> AHVVTDNCIKCKYTDCVEVCPVDCFYEGPNFLVIHPDECIDCALCEPECPAQAIFSED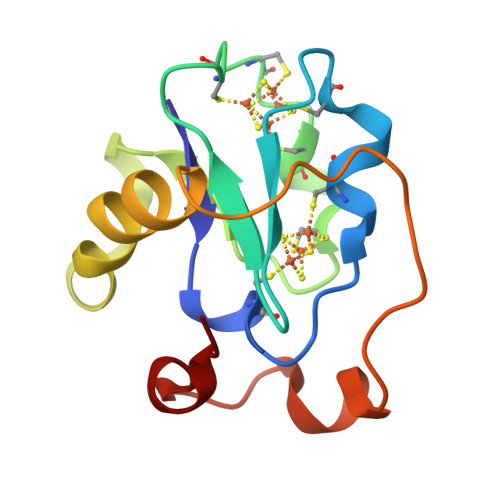EVPEDMQEFIQLNAELAEVWPNITEKKDPLPDAEDWDGVKGKLQHLER> MSEMSYLEKLLDGVEVEWLPLGEITKYEQPTKYLVKAKDYHDTYTIPVLTAGKTFILGYTNETHGIYQASKAPVIIFDDFTTANKWVDFDFKAKSSAMKMVTSCDDNKTLLKYVYYWLNTLPSEFAEGDHKRQWISNYSQKKIPIPCPD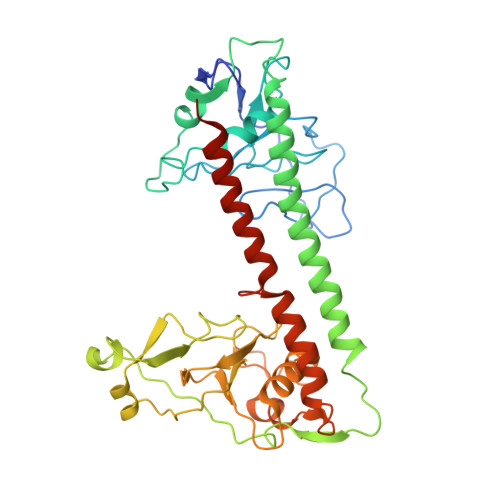NPEKSLAIQSEIVRILDKFTALTAELTAELNMRKKQYNYYRDQLLSFKEGEVEWKTLGEIGKWYGGGTPSKNKIEFWENGSIPWISPKDMGRTLVDSSEDYITEEAVLHSSTKLIPANSIAIVVRSSILDKVLPSALIKVPATLNQDMKAVIPHENILVKYIYHMIGSRGSDILRAAKKTGGSVASIDSKKLFSFKIPVPNINEQQRIVEILDKFDTLTNSITEGLPREIELRQKQYEYYRDLLFSFPKPETVSN>GSAKDPMPGAVDFKERISRQRPHDRETYGHAGNTDLQDIVYQLESDRGRIVNSAAVRRLQQKTQVFPLERNAAVRSRLTHSLEVQQTGRFIVRTLFRQLGPRAAEVGLDGLEGALESLVEMACLMHDVGNPPFGHFGEYAINDWFERNLDALFERRVPPGQGDGLLQQRMLTDLKHFEGNAQAIRLVVKLLRLNLTYTQTAGLLKYVRPAYEPKPDKAAANHYLNKKPGFYLSEEAFVDELRQVLGMRPGTRHPVAYIMEAADDISYCLADIEDSVEKGILDIRQLADLLVKKFAVHHSPDAPIPGDADNMSFQRMVDYSLEKAEREPINKVSEFFIRLRVKMIHPLVQHAAQQFIDNLEAVHAGTLGRALMEDGSLPHAIVQTFKDVAMEWVFCHPEVETLELQGYRIIQGLLDFYAPLLRLPAEEFQALAEGRQAAAPHPQLLVRRLPSQQIKAYLEAMKGVAEDPLQR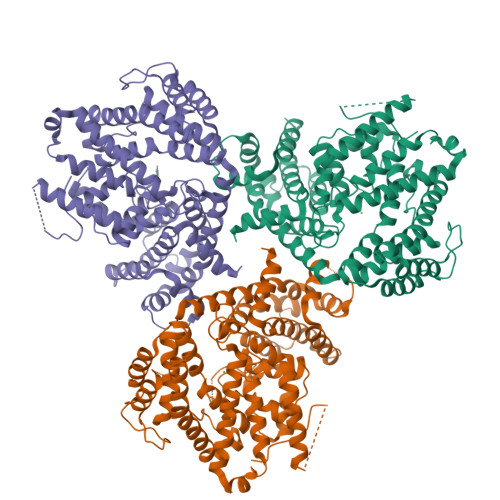QWEFYHRCRMLQDFVSGMTDQHAQDEYRALSAL[3x]> ETGESPPVFIKKPVDQIGVSGGVASFVCQATGDPKPRVTWNKKGKKVNSQRFETIEFDESAGAVLRIQPLRTPRDENIYECVAQNPHGEVTVHAKLTVLREDQLPPGFPNIDMGPQLKVVERTRTATMLCAASGNPDPEITWFKDFLPVDPS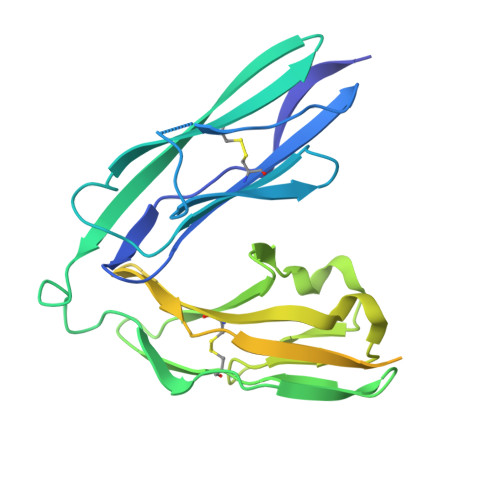TSNGRIKQLRSGGLQIESSEETDQGKYECVASNSAGVRYSSPANLYVRVRRVAPRFSILPVSHEIMPGGNVNITCVAVGSPMPYVKWMQGAEDLTPEDDMPVGRNVLELTDVKDSANYTCVAMSSLGVIEAVAQITVKSKGHHHHHH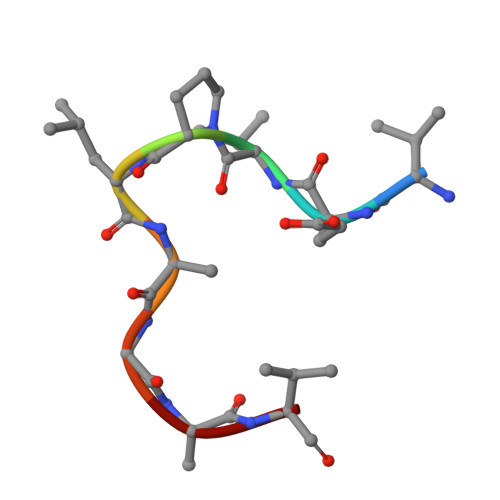> VEVPLAGAV(3S)-N-[(1-benzothiophen-5-yl)methyl]-1-{2-[4-(trifluoromethyl)phenyl]-2H-pyrazolo[3,4-d]pyrimidin-4-yl}piperidine-3-carboxamide | C27 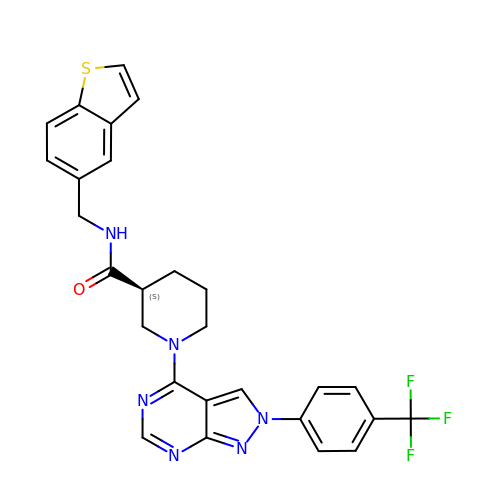H23 F3 N6 O S | RPVUYLFRBVBINJ-IBGZPJMESA-N6-ACETYL-8-CYCLOPENTYL-5-METHYL-2-[(5-PIPERAZIN-1-YLPYRIDIN-2-YL)AMINO]PYRIDO[2,3-D]PYRIMIDIN-7(8H)-ONE 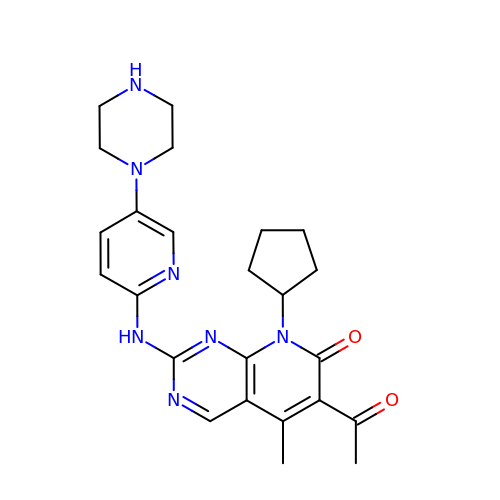| C24 H29 N7 O2 | AHJRHEGDXFFMBM-UHFFFAOYSA-N>GQDMVSPPPPIADEPLTVNTGIYLIECYSLDDKAETFKVNAFLSLSWKDRRLAFDPVRSGVRVKTYEPEAIWIPEIRFVNVENARDADVVDISVSPDGTVQYLERFSARVLSPLDFRRAPFDSQTLHIYLIVRSVDTRNIVLAVDLEKVGKNDDVFLTGWDIESFTAVVKPANFALEDRLESKLDYQLRISRQYFSYIPNIILPMLFILFISWTAFWSTSYEANVTLVVSTLIAHIAFNILVETNLPKTPYMTYTGAII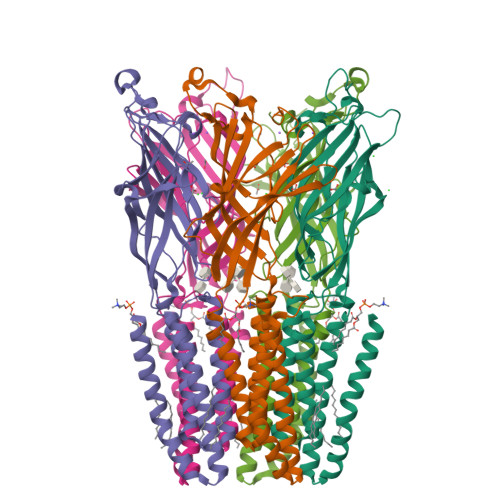FMIYLFYFVAVIEVTVQHYLKVESQPARAASITRASRIAFPVVFLLANIILAFLFFGF[5x]> ARSTNTFNYATYHTLDEIYDFMDLLVAQHPELVSKLQIGRSYEGRPIYVLKFSTGGSNRPAIWIDLGIHSREWITQATGVWFAKKFTENYGQNPSFTAILDSMDIFLEIVTNPNGFAFTHSENRLWRKTRSVTSSSLCVGVDANRNWDAGFGKAGASSSPCSETYHGKYANSEVEVKSIVDFVKNHGNFKAFLSIHSYSQLLLYPYGYTTQSIPDKTELNQVAKSAVAALKSLYGTSY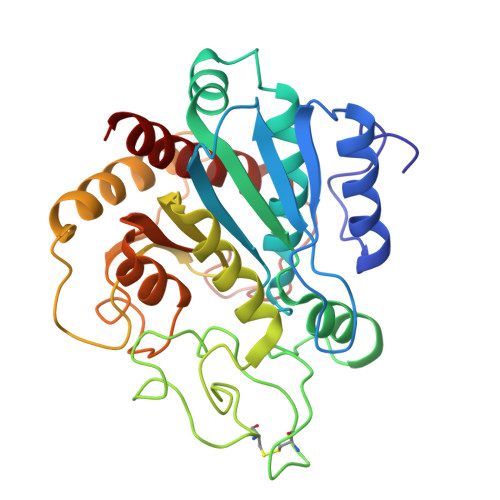KYGSIITTIYQASGGSIDWSYNQGIKYSFTFELRDTGRYGFLLPASQIIPTAQETWLGVLTIMEHTVNN>SNAMIYPDETMLYAPVEWHDCSEGYTDIRYEKSTDGIAKITINRPQVRNAFRPLTVKEMIQALADARYDDNVGVIILTGEGDKAFCAGGDQKVRGDYGGYQDDSGVHHLN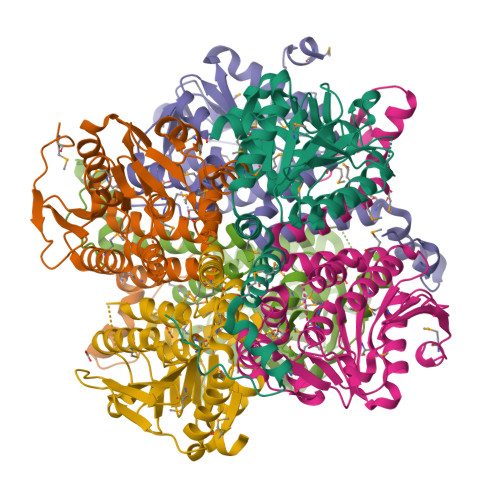VLDFQRQIRTCPKPVVAMVAGYSIGGGHVLHMMCDLTIAAENAIFGQTGPKVGSFDGGWGASYMARIVGQKKAREIWFLCRQYDAQQALDMGLVNTVVPLADLEKETVRWCREMLQNSPMALRCLKAALNADCDGQAGLQELAGNATMLFYMTEEGQEGRNAFNQKRQPDFSKFKRNP[6x]>[2x]GAMVIRDENYFTDKYELTRTHSEVLEAVKVVKPGKTLDLGCGNGRN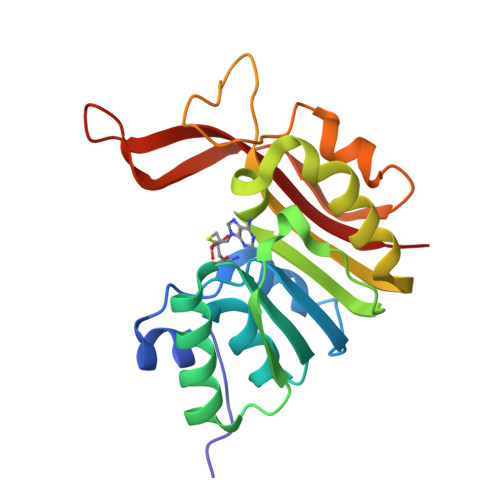SLYLAANGYDVDAWDKNAMSIANVERIKSIENLDNLHTRVVDLNNLTFDRQYDFILSTVVLMFLEAKTIPGLIANMQRCTKPGGYNLIVAAMDTADYPCTVGFPFAFKEGELRRYYEGWERVKYNEDVGELHRTDANGNRIKLRFATMLARKK> MSMNRQEISDLCVKSLEGRMVGTEAQNIENGNAFYRYFFTNFPDLRVYFKGAEKYTADDVKKSERFDKQGQRILLACHLLANVYTNEEVFKGYVRETINRHR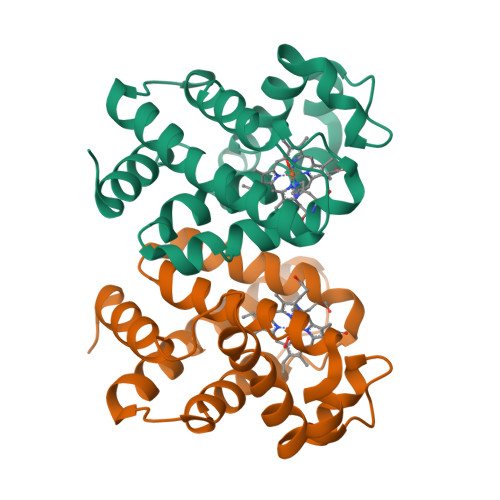IYKMDPALWMAFFTVFTGYLESVGSLNDQQKAAWMALGKEFNAESQTHLKNSNLPHV> MGLISDADKKVIKEEFFSKMVNPVKLIVFVRKDHCQYCDQLKQLVQELSELTDKLSYEIVDFDTPEGKELA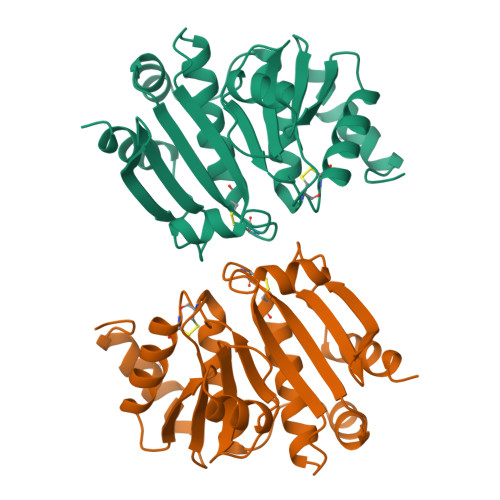KRYRIDRAPATTITQDGKDFGVRYFGLPAGHEFAAFLEDIVDVSREETNLMDETKQAIRNIDQDVRILVFVTPTCPYCPLAVRMAHKFAIENTKAGKGKILGDMVEAIEYPEWADQYNVMAVPKIVIQVNGEDRVEFEGAYPEKMFLEKLLSALS> MASMSVSTASTEMSVRKIAAHMKSNPNAKVIFMVGAGISTSCGIPDFRSPGTGLYHNLARLKLPYPEAVFDVDFFQSDPLPFYTLAKELYPGNFRPSKFHYLLKLFQDKDVLKRVYTQNIDTLERQAGVKDDLIIEAHGSFAHCHCIGCGKVYPPQVFKSKLAEHPIKDFVKCDVCGELVKPAIVFFGEDLPDSFSETWLNDSEWLREKITTSGKHPQQPLVIVVGTSLAVYPFASLPEEIPRKVKRVLCNLETVGDFKANKRPTDLIVHQYSDEFAEQLVEELGWQEDFEKILTAQ;> KGG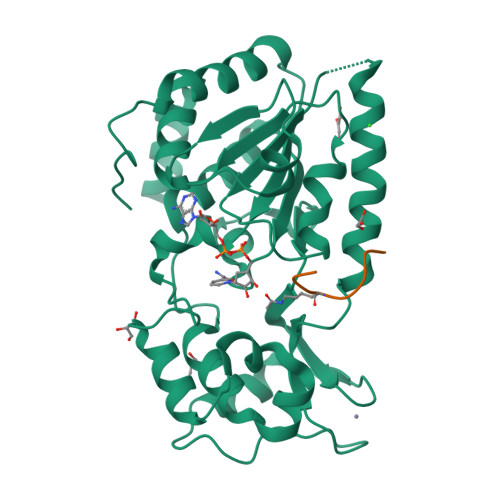AKRHRKI> QAQITGRPEWIWLALGTALMGLGTLYFLVKGMGVSDPDAKKFYAITTLVPAIAFTMYLSMLLGYGLTMVPFGGEQNPIYWARYADWLFTTPLLLLALALLVDADQGTILALVGADGIMIGTGLVGALTKV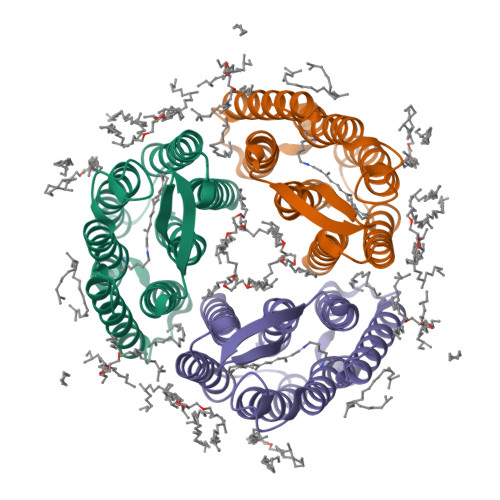YSYRFVWWAISTAAMLYILYVLFFGFTSKAESMRPEVASTFKVLRNVTVVLWSAYPVVWLIGSEGAGIVPLNIETLLFMVLDVSAKVGFGLILLRSRAIFGEAEAPEPSAGDGAAATSD Botulinum neurotoxins (BoNTs) are bacterial toxins produced predominantly by Clostridium botulinum. The heavy chain contains two domains: the receptor-binding domain (HC) which is responsible for targeting neuronal cells at the presynaptic neuromuscular junction, and the translocation domain (HN) which transfers the LC across the endosomal membrane within the cytosol. BoNT/B, /G, and /DC instead bind to either Synaptotagmin I or II (SytI or SytII). BoNT/B2 from Clostridium botulinum strain 111 was first identified in a case of infant botulism and initial characterization found its toxicity to be approximately 10 times lower than that of BoNT/B1.

Instead, only crystals containing HC/B2 in complex with hSytI were produced in the space group P212121, which diffracted to a resolution of 2.5 Å. Electron density can be seen for residues 46 to 59 of hSytI but not for residues either side, indicating some flexibility. There are four residue differences between BoNT/B1 and BoNT/B2 which are in close proximity to the bound Syt peptide: P1117S, P1197N, E1191K, S1199Y. The change from two hydrophobic proline residues to two polar residues (Ser and Asn) is likely to result in a significant change in binding affinity as both of these residues are found neighboring the conserved and central Phe residues of Syt, known to be key elements of the hydrophobic binding mechanism. In BoNT/B2, this loss of hydrophobic interaction is replaced by electrostatic contacts between S1117 and N1197 and the peptide backbone of hSytI. Conversely, the change from S1199 in BoNT/B1 to Y1199 in BoNT/B2 would be expected to provide increased affinity for the peptide via aromatic interactions with F47. Here we observed that both N1197, via its hydrogen bond with F47, and Y1199 contribute to shifting the N-terminal part of the hSytI backbone slightly further away (1Å) compared to its position when bound to B1. In BoNT/B2 however, substitution of a negative (Glu) to a positive (Lys) side chain at position 1191 likely decreases the affinity of B2 for its receptor. Although the backbone of the hSytI peptide occupies a position similar to the one when bound to B1, we identified several amino acid substitutions that cause a loss of hydrophobic interactions between B2 and Syt, thus affecting the overall affinity for the receptor. In B2, the presence of Y1199 is not enough to compensate for the loss of affinity resulting from substitutions P1117S, P1197N, and E1191K.

> SHMNSEILNNIILNLRYRDNNLIDLSGYGANVEVYDGVELNDKNQFKLTSSTNSEIRVTQNQNIIFNSMFLDFSVSFWIRIPKYKNDGIQNYIHNEYTIINCIKNNSGWKISIRGNRIIWTLTDINGKTKSVFFEYSIREDISDYINRWFFVTITNNSDNAKIYINGKLESNIDIKDIGEVIANGEIIFKLDGDIDRTQFIWMKYFSIFNTELSQSNIKEIYKIQSYSEYLKDFWGNPLMYNKEYYMFNAGNKNSYIKLKKDSSVGEILTRSKYNQNSNYINYRNLYIGEKFIIRRKSNSQSINDDIVRKEDYIYLDFFNSNREWRVYAYKDFKEEEKKLFLANIYDSNEFYKTIQIKEYDEQPTYSCQLLFKKDEESTDEIGLIGIHRFYESGIVLKDYKNYFCISKWYLKEVKRKPYNPNLGCNWQFIPKDEGWIE;> GEGKEDAFSKLKEKFMNELHK>MIHLRPDSTAYARSAAVSANPAVGGYVTPDNTVLEGQNPSALVQAMQKPVASVTDSFKATLSESIGAKALRGVEYASIPTEAGFEPSKALGDSVSQYTADELEFLSDARSSAELAQRRSQVQDTRNNYDAMGQNMLTTVAASMLDVDMVIGGGVGALSKVSRATRLAVGLSANAALLGTASYGGTITPLDVVGTSVGIAMSAIPGIRKVAKAEQVQQGAVRGGVNAAEDAAGTVVPPKDVTVPPVREVPEVQPIKTVADEDYPKIDIDTYSNKEHIEVGRTGGAKTGSLKTTVQNAVLAVTALGDDLPEGVRALGRALGASLEADADVPVVFRSRTGANAQARSAVITEAETGATRAEIFNPAVGGTLSDHVRGMSTYEKTILLHEAAHAKTGRSIRAVESGAVSDGVVYEAVQRIKEIQWYVKANVELPPLGKGAKYNVDYGLSDTHEFISQLFNSEHFRDALRSVKMPGSDGTLLSNLMKRVVTLFTGKAPEGNAFDATLQAFDNLLSQ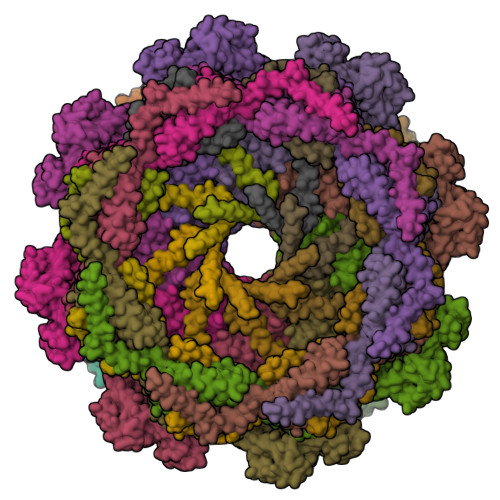PTTPADVFLNAPKATPDLQSKVLQAPNVIEMNNKVMGALNRNFSLYERLKSFGYKASTLADQLVVDATGTEANSAAHHARAAHLASNVSIVQVDDAFRQALSADWPLVQRLRHPVLYREAQRDLSQKVYQQLAENHDRFLKGQSIQPSNDPRVNSMVDAFVNSNWAKDELARVKGAGINGADAVRESPYYLPRQHSGNKLNDFMRNNRQVTKDDIVGMYTEQFSRMFQQNGITPETARKLGAKMFDNMQDQAAHVQGYRQSIAGMSYDDIENTLEALGASDPTITAFLDAVKGSGEQANKVRNLRGRAEFDMTAQYTTKSGDMISPSMFVNNDVMGLMEGYSRRMSGRVGLAKAGFPDLRDAVKAIDEAAAEAQDPAAALHAFDNTMNQILGYPTGEDVPDILRSASIIGGALNLANSGIYQLADMSLMLQQFGITKTLKAFGSTAFGRNAMDVAKSAEFGSRLQDVIEARHVLSGKYRSVLTHLEDNRDIGSLGVAHRYVQQMGQGTRFVNGMEFIRRGQAKLVSGLIADTVDDAIAGNASAVTAMERFGLNQQLLDELRKATAANPDMRKWPDSVRMDIEAVTHNMADSIVLENRLGEIPAWMQFSSVGKVILPYMTFVAGAWNKILRRTAKLDGATGVAIALAYQMPLVTLSSATSIAISGKPVTPESVAQRALVQVPMMSWAGFAVDFWANGASNNLAALALVDRMHAAMSSIASGETNPESLIKAVPFLSILPGMRLMGASLADDDE[4x];>MPVRQPTQGGVQVPGLTGYQSAGVAQPVYRAPQEEAQGVSQFWQNLLPASVKTAQAAQQTASAKGYLEGQQDSQQGREKQVRNFFTKEAYEQGYNSASVNSALASFQLGLQNTAQQYVNSGKTPEEFNVHVQQQTNQLLQEAGAQGLNLNDKDWQAWLGSVEHSRNTANASYQDLNLKRAAVLQEQSWGARGNAAIADFVTAQQSGDTEQALQNVNSFISSVTHDDSITAENKIKYTSQFVVNAFANANSTGDMQALTGYVQSLSEFKNMPTDVQTQIMGSAQQYYQQRASDESVQLYEYNSRVNSVTDYKTLNEAYPMAQYIGTVMQAVQQKKLSPGTGYGMVDAESQRRLKMQKAEQGQLAYTNGVTISDIAAGTGESLDKVKGELTKMYATIGQGYSGGGLQLMQRGLKSGAQDITGVGIEMMQQDAQSLSGIDWRNLKTDADGKPLYPAAVVGSLGNLQAAYQSALAAGNQVQANQLLSGLPDPVVYGIRQNVDARDLADVVGKRAQDIASGKVLALPANMPADVSITQADVTAGIFDLGLGKDARNRNMLGIQSWVFTSDADEKAAQARVSQVNSAMNNEYVYNQQRGSLPALVGDDLKSWLMGKVASRTVRVKDGTDNGALLVLPEVGDKQKVFGSTDNGIIESALTESVTNFKKQYPQATTVQMDYDPLTQELIFQGVNAENQLGTTRASIPAADFRNTVRGVQNTLTQNGSGTTQGNLNVPGAGFVSFNAGNSFGIQKNVVMGAVNQLVSYEGYTPSKGFSVLGVHPTTGAKLNEDKYVKQATDTPQVAADKFNMYLNDKVYPLVMPKMEQYKNLPGYIQNNIYNALVETTYHSGNSDVFDKYIQTALYGNVQEIPTFKDTPLFKDAGAGSRRNVDRYQLLGSLVTYRTNNPNLSK[8x];>MIWMFAAAAAQMIQGGLQYAQDAKNQRRQNKADQKYNEAVRSASARQITEINTQRSVSRAQTAQALDAARRQGAGESSARNLQAAATDTMGASVEQNLQEVGVQLAAAEGNLMQNAELTELSLDSSVMNTVDQARNSIRELSNPLGTDWAATGSAVGQIGTSMVANKLGGQGWFGGNSGTQQPAPISQAAPPTRSNNLSTRLNV[8x]>[2x]CGIVGIAGVMPVNQSIYDALTVLQHRGQDAAGIITIDANNCFRLRKANGLVSDVFEARHMQRLQGNMGIGHVRYPTAGSSSASEAQPFYVNSPYGITLAHNGNLTNAHELRKKLFEEKRRHINTTSDSEI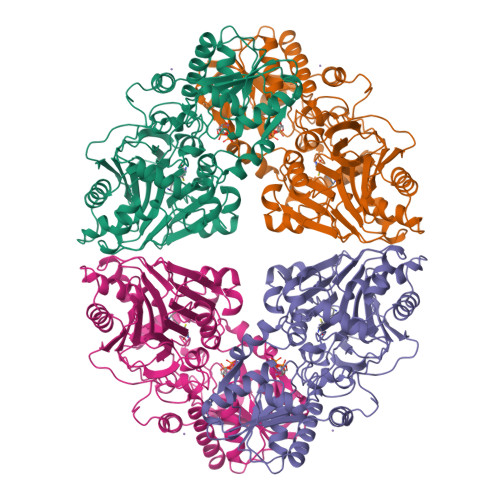LLNIFASELDNFRHYPLEADNIFAAIAATNRLIRGAYACVAMIIGHGMVAFRDPNGIRPLVLGKRDIDENRTEYMVASESVALDTLGFDFLRDVAPGEAIYITEEGQLFTRQCADNPVSNPCLFEYVYFARPDSFIDKISVYSARVNMGTKLGEKIAREWEDLDIDVVIPIPETSCDIALEIARILGKPYRQGFVKNRYVGRTFIMPGQQLRRKSVRRKLNANRAEFRDKNVLLVDDSIVRGTTSEQIIEMAREAGAKKVYLASAAPEIRFPNVYGIDMPSATELIAHGREVDEIRQIIGADGLIFQDLNDLIDAVRAENPDIQQFECSVFNGVYVTKDVDQGYLDFLDTLRNDDAKAVQRQNEVENLEMHNEG> MNVYDDVLDATVVSHSLATHFTTSDYEELLVVRTNILSVYRPTRDGKLYLTDEFKFHGLITDIGLIPQKDSPLSCLLLCTGVAKISILKFNTLTNSIDTLSLHYYEGKFKGKSLVELAKISTLRMDPGSSCALLFNNDIIAFLPFHVNKNDDDEEEEDEDENIDDSELIHSMNQKSQGTNTFNKRKRTKLGDKFTAPSVVLVASELYEGAKNIIDIQFLKNFTKPTIALLYQPKLVWAGNTTISKLPTQYVILTLNIQPAESATKIESTTIAFVKELPWDLHTIVPVSNGAIIVGTNELAFLDNTGVLQSTVLLNSFADKELQKTKIINNSSLEIMFREKNTTSIWIPSSKSKNGGSNNDETLLLMDLKSNIYYIQMEAEGRLLIKFDIFKLPIVNDLLKENSNPKCITRLNATNSNKNMDLFIGFGSGNALVLRLNNLKSTIETREAHNPSSGTNSLMDINDDDDEEMDDLYADEAPENGLTTNDSKGTVETVQPFDIELLSSLRNVGPITSLTVGKVSSIDDVVKGLPNPNKNEYSLVATSGNGSGSHLTVIQTSVQPEIELALKFISITQIWNLKIKGRDRYLITTDSTKSRSDIYESDNNFKLHKGGRLRRDATTVYISMFGEEKRIIQVTTNHLYLYDTHFRRLTTIKFDYEVIHVSVMDPYILVTVSRGDIKIFELEEKNKRKLLKVDLPEILNEMVITSGLILKSNMCNEFLIGLSKSQEEQLLFTFVTADNQIIFFTKDHNDRIFQLNGVDQLNESLYISTYQLGDEIVPDPSIKQVMINKLGHDNKEEYLTILTFGGEIYQYRKLPQRRSRFYRNVTRNDLAITGAPDNAYAKGVSSIERIMHYFPDYNGYSVIFVTGSVPYILIKEDDSTPKIFKFGNIPLVSVTPWSERSVMCVDDIKNARVYTLTTDNMYYGNKLPLKQIKISNVLDDYKTLQKLVYHERAQLFLVSYCKRVPYEALGEDGEKVIGYDENVPHAEGFQSGILLINPKSWKVIDKIDFPKNSV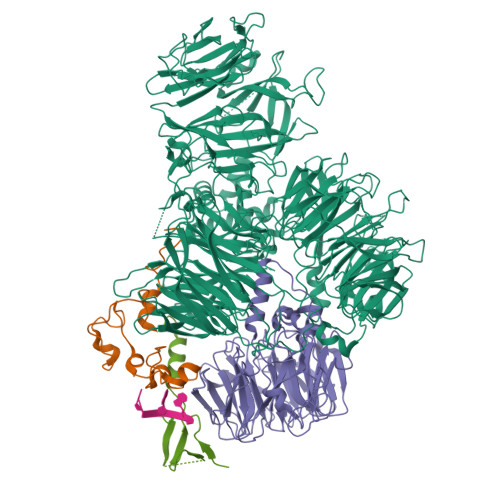VNEMRSSMIQINSKTKRKREYIIAGVANATTEDTPPTGAFHIYDVIEVVPEPGKPDTNYKLKEIFQEEVSGTVSTVCEVSGRFMISQSQKVLVRDIQEDNSVIPVAFLDIPVFVTDSKSFGNLLIIGDAMQGFQFIGFDAEPYRMISLGRSMSKFQTMSLEFLVNGGDMYFAATDADRNVHVLKYAPDEPNSLSGQRLVHCSSFTLHSTNSCMMLLPRNEEFGSPQVPSFQNVGGQVDGSVFKIVPLSEEKYRRLYVIQQQIIDRELQLGGLNPRMERLANDFYQMGHSMRPMLDFNVIRRFCGLAIDRRKSIAQKAGRHAHFEAWRDIINIEFSMRSLCQGK;> MSLIHPDTAKYPFKFEPFLRQEYSFSLDPDRPICEFYNSREGPKSCPRGPLCPKKHVLPIFQNKIVCRHWLRGLCKKNDQCEYLHEYNLRKMPECVFFSKNGYCTQSPDCQYLHIDPASKIPKCENYEMGFCPLGSSCPRRHIKKVFCQRYMTGFCPLGKDECDMEHPQFIIPDEGSKLRIKRDDEINTRKMDEEKERRLNAIINGEV;> MDGHNQNQYQNQNQIQQSQQPPLKKYVTQRRSVDVSSPYINLYYNRRHGLPNLVVEPETSYTIDIMPPNAYRGRDRVINLPSKFTHLSSNKVKHVIPAIQWTPEGRRLVVATYSGEFSLWNASSFTFETLMQAHDSAVTTMKYSHDSDWMISGDADGMIKIWQPNFSMVKEIDAAHTESIRDMAFSSNDSKFVTCSDDNILKIWNFSNGKQERVLSGHHWDVKSCDWHPEMGLIASASKDNLVKLWDPRSGNCISSILKFKHTVLKTRFQPTKGNLLMAISKDKSCRVFDIRYSMKELMCVRDETDYMTLEWHPINESMFTLACYDGSLKHFDLLQNLNEPILTIPYAHDKCITSLSYNPVGHIFATAAKDRTIRFWTRARPIDPNAYDDPTYNNKKINGWFFGINNDINAVREKSEFGAAPPPPATLEPHALPNMNGFINKKPRQEIPGIDSNIKSSTLPGLSI;> MSSTIFYRFKSQRNTSRILFDGTGLTVFDLKREIIQENKLGDGTDFQLKIYNPDTEEEYDDDAFVIPRSTSVIVKRSPAIKSFSVHSRLKGNVGAAALGNATRYVTGRPRVLQKRQHTATTTANVSGTTEEERIASMFATQENQWEQTQEEMSAATPVFFKSQTNKNSAQENEGPPPPGYMCYRCGGRDHWIKNCPTNSDPNFEGKRIRRTTGIPKKFLKSIEIDPETMTPEEMAQRKIMITDEGKFVVQVEDKQSWEDYQRKRENRQIDGDETIWRKGHFKDLPDDLKCPLTGGLLRQPVKTSKCCNIDFSKEALENALVESDFVCPNCETRDILLDSLVPDQDKEKEVETFLKKQEELHGSSKDGNQPETKKMKLMDPTGTAGLNNNTSLPTSVNNGGTPVPPVPLPFGIPPFPMFPMPFMPPTATITNPHQADASPKK2-(((R)-2,3-DIHYDROXYPROPYL)PHOSPHORYLOXY)-N,N,N-TRIMETHYLETHANAMINIUM 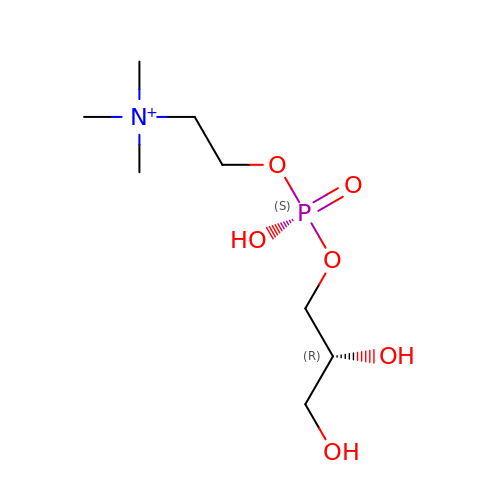| C8 H21 N O6 P | SUHOQUVVVLNYQR-MRVPVSSYSA-O> XVNAKQXHRIXKRRQARAKLX;> GPSFREQDIYLPIANVARIMKNAIPQTGKIAKDAKECVQECVSEFISFITSEASERCHQEKRKTINGEDILFAMSTLGFDSYVEPLKLYLQKFRE;> GPMEEIRNLTVKDFRVQELPLARIKKIMKLDEDVKMISAEAPVLFAKAAQIFITELTLRAWIHTEDNKRRTLQRNDIAMAITKFDQFD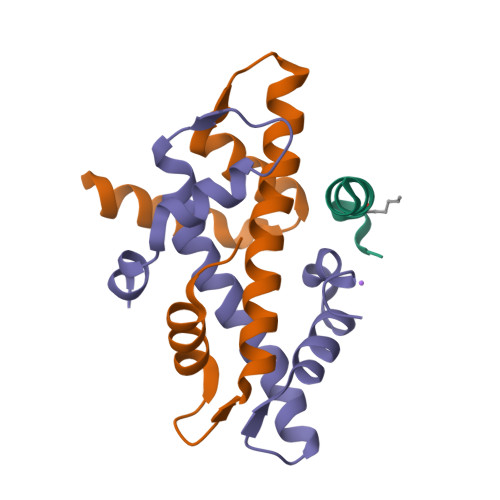FLIDIVPR>[8x]AMKQEQMRLANQLCFSAYNVSRLFAQFYEKKLKQFGITYSQYLVLLTLWEENPQTLNSIGRHLDLSSNTLTPMLKRLEQSGWVKRERQQSD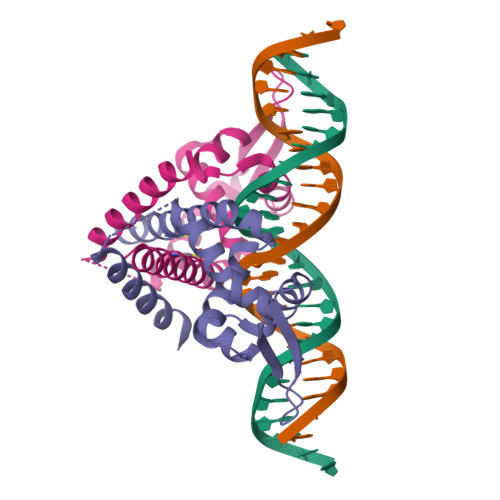KRQLIITLTDNGQQQQEAVFEAISSCLPQEFDTTEYDETKYVFEELEQTLKHLIEK>[2x]GPGSISLGDLHGNAIKLIHFLFRHKIIKFKTEIINFHEAYQQFVTIYEQYDDMVQEYLEIRTLLQLIQIKITNA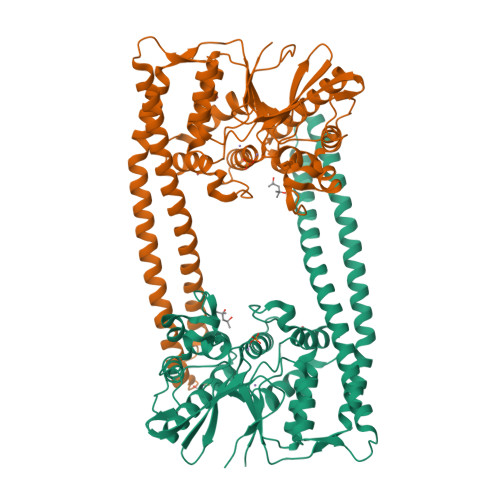QQRILDIEQKLSLATDHQKEFSQSLLQLKKPIEANLQMAEKSKAGLEEKLSGLKTRLPSCIERFNKFMTQIEINDIKTLIRLLGDEVADRGSCDYFTLRILDFLYQNQIAIKIILSNHGYEFIHAYEKLVVGQPFKPKGYIGDIQIKSFWGLQLLLEQSVITEEELRSLVERAYKPTLKIIDYSLSEDGITLYSHAPIRFDSIRMAASQLGVTYNDSTKEALAETIDQLNAQLQIYMKNNMLHLLFENNEINDPTNMTDEERNASPLIYLVWNRWNESKEVENARPGKYNGYFVTYVHGHDPFQSPLTYVYNLDTLCGKYSRVGEEEQINKAFQFLTENR N~2~-[(2H-1,3-benzodioxol-5-yl)methyl]-N-hydroxy-N~2~-[(4-methoxyphenyl)sulfonyl]-3-thiophen-2-yl-D-alaninamide 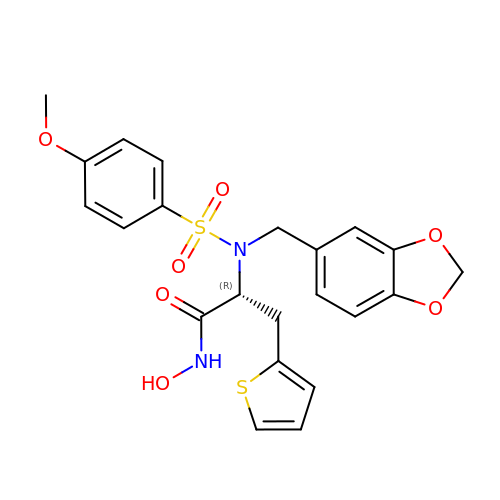| C22 H22 N2 O7 S2 | PGEHBYYTLWHQOM-LJQANCHMSA-N>MGSSHHHHHHSSGRENLYFQGMKLATLKDSTRDGKLVVVSKDLTRCSEVGHIARTLQAALDDWAHAGPRLERVAEGIETGAQPTMRFHEHDAASPLPRAFQWADGSAYVNHVELVRKARNAEMPASFWTDPLIYQGGSDSFLGPRDPILMADDAWGIDMEGEAAVIVDDVPMGATLDEAKAAIRLVMLVNDVSLRGLIPGELAKGFGFYQSKPSSAFSPVAVTPEELGEAWDGGKLHLPLHVDLNGEPFGRANAGIDMTFDFPQLIVHAARTRPLSAGTIIGSGTVSNKLEGGPGRPVSEGGAGYSCIAELRMIETIEGGAPKTQFLK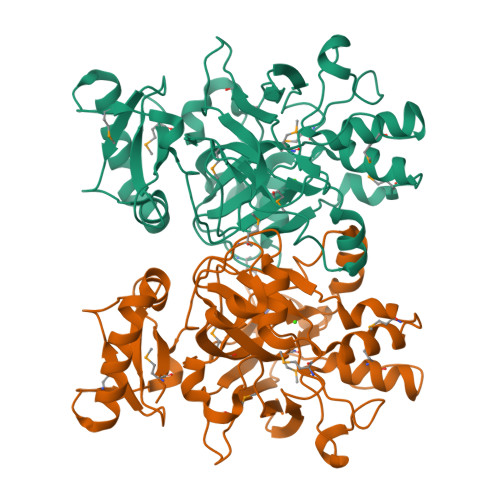FGDVVRIEMKDRTGHSIFGAIEQKVGKYERG[4x]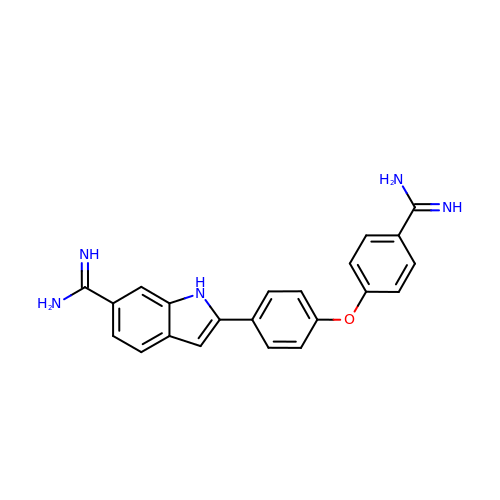2-[4-(4-carbamimidoylphenoxy)phenyl]-1H-indole-6-carboximidamide | C22 H19 N5 O | OSSYTOVYXCAWPG-UHFFFAOYSA-N>[2x]GMTVTDNPADTAGEATAGRPAFVSRSVLVTGGNRGIGLAIARRLAADGHKVAVTHRGSGAPDDLFGVQCDVTDSAAVDRAFKEVEEHQGPVEVLVANAGISKDAFLMRMTEERFEEVINTNLTGAFRCAQRASRTMQRKRFGRIIFIGSVSGMWGIGNQANYAAAKAGLIGMARSISRELAKAGVTANVVAPGYIDTEMTRALDERIQAGALDFIPAKRVGTAEEVAGAVSFLASEDASYIA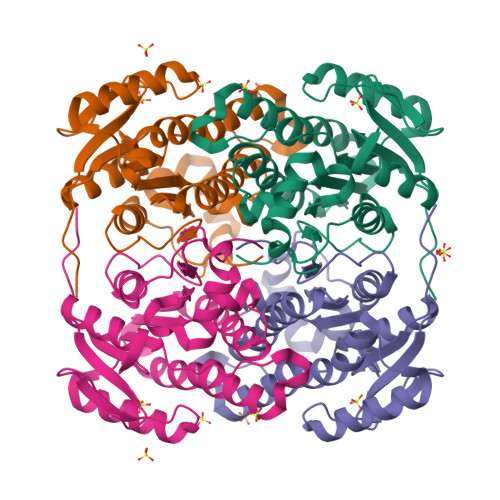GAVIPVDGGMGMGH Glutathione, the tri-peptide γ-L-glutamyl-cysteinyl-glycine, is the main low molecular weight thiol antioxidant in both plant and animal cells, often present at millimolar concentrations in vivo. It is synthesised in a two-step, ATP-dependent, process: glutamate-cysteine ligase (GCL) catalyses the formation of γ-glutamylcysteine (γ-EC) from glutamate and cysteine, followed by the addition of glycine by glutathione synthetase (GS) to form glutathione. Cyst nematodes have exploited a series of gene gain events to redeploy glutathione synthetase-like enzymes during parasitism, within the syncytial feeding cell formed in the host root. The most recent expansion has been coupled with a diversification of structure and biochemical function that has given rise to enzymes that are introduced into the host cell, and likely possess novel substrate specificities.

To explore the catalytic capacity of nematode GS-like genes, the G. pallida representative of Clade 1 (Gpa-gss1), one representative from Clade 2 (Gpa-gss5) and a number from Clade 3 (Gpa-gss12, Gpa-gss17, Gpa-gss22, Gpa-gss24 and Gpa-gss30) were heterologously expressed in, and their proteins purified from, bacteria. Remarkably, each stage of the evolutionary process that gave rise to GS-like effectors has witnessed at least a 10-fold reduction in apparent glutathione synthetic rate, such that Clade 3 GS-like proteins have not retained canonical enzyme activity. In contrast, none of the Clade 3 GS-like effectors accepted any of the tested terminal amino acid substrates in combination with the γ-EC backbone. Comparison between Gpa-GSS22-open and–closed reveals a functioning ATP grasp fold. Residues in the ATP binding pocket of St-GSS1 are highly conserved in sequence and position in the Gpa-GSS22 structure (13/15 residues), and similarly conserved in sequence across G. pallida Clade 3 (structure guided alignment, ~12/15, n = 24). In contrast, there is considerably more variation in the di-peptide binding pocket of G. pallida GS-like effectors, yet, this variation is not evenly distributed around the pocket. However, the glutamate of the di-peptide is exclusively coordinated by interactions with charged side chains of residues in the binding pocket (R, E, 2xQ, N, and Y). All six of these positions are substituted in Gpa-GSS22 and Gpa-GSS30, thus suggesting that the lack of canonical activity is because γ-EC is not accepted despite the potential for cysteine to be accommodated. Variability in the glutamate portion of the di-peptide binding pocket is ubiquitous in G. pallida Clade 3 GS: of the 24 GS-like effectors there are 21 different amino acid compositions in these 6 positions, not one of which is canonical.

>[2x]MNCDNAKFIIFFFFIIFLCANFAVCNELEDYVEKSVNSETKLHKLADFAIDWAHNNGLILRTKQFLNKSDVAEFAPVSLLPSPFPRHAFEKAVAVHEALQLLYFRVACDYEFMMDAYKDVVNTDNHLRQLVNIIKDAHKQGIKQPTTLLIMRADYMLNTLNSKGNDDEYELKQVEVNTGAIGGLGIDRRTTELHRQMLRKVGMDTSNSPANNGDSNMIESLFMAWEAFGNKNALFVFLSHERLQYKFELRNIQCQLEELSNGQMKVEYVSLKAGYEQLKLGEDYSLLLNGEIVGVVYSTISALGHQANAREMEARRTIELSNAIKAPSLAIAISSSKKIQQLLTTPGTLERFFPSATEADKVAAIRETFTGLWGLEKSDDQTERRIKDAIENPANYVLKSNGECGGNNFYDEALAEKLRTMPQAERASHILMQKLIPMATKNYFLRPFHEPKLNVVVGELGVNGTLLGNLRDQSVRHNVQSGHLLRTKLREANEGGISVGTGVGDSPYLF N~5~-{3-[(1-methylethyl)sulfanyl]propanimidoyl}-L-ornithine | C11 H23 N3 O2 S | 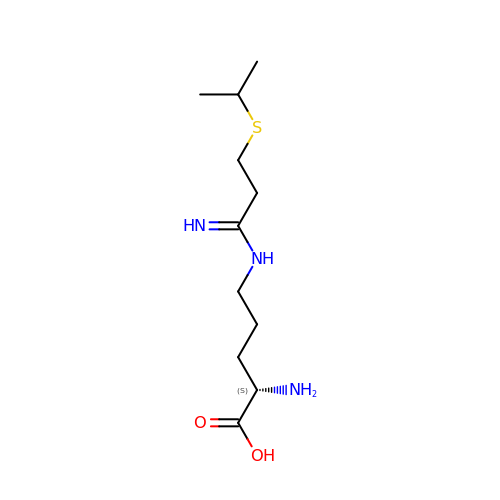YRGYNHWJLFBYTL-VIFPVBQESA-N>MPKRGKKGAVAEDGDELRTEPEAKKSKTAAKKNDKEAAGEGPALYEDPPDQKTSPSGKPATLKICSWNVDGLRAWIKKKGLDWVKEEAPDILCLQETKCSENKLPAELQELPGLSHQYWSAPSDKEGYSGVGLLSRQAPLKVSYGIGDEEHDQEGRVIVAEFDSFVLVTAYVPNAGRGLVRLEYRQRWDEAFRKFLKGLASRKPLVLCGDLNVAHEEIDLRNPKGNKKNAGFTPQERQGFGELLQAVPLADSFRHLYPNTPYAYTFWTYMMNARSKNVGWRLDYFLLSHSLLPALCDSKI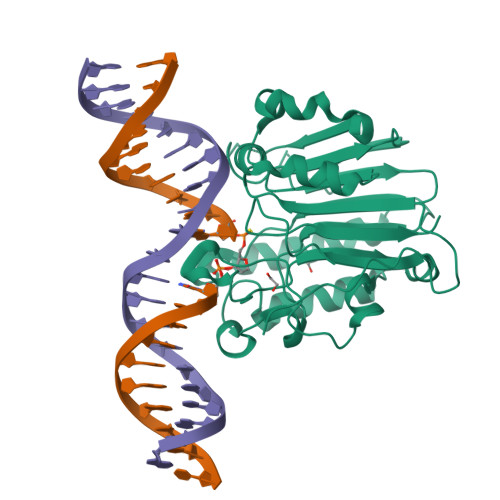RSKALGSDHCPITLYLAL[2x]BgaA is specific for galactose β-1,4-linked to glucose or GlcNAc [lactose or N-acetyllactosamine (LacNAc) motifs, respectively] found in glycoconjugates. The N-terminal region of BgaA comprising amino acid residues 138–993 has amino acid sequence identity with GH family 2 enzymes. Through detailed structural and functional analyses the molecular basis for the catalytic specificity of BgaA is defined and this activity is demonstrated as critical for the ability of pneumococci to utilize complex N-linked glycans as a carbon source and protect the bacterium from opsonophagocytic killing. Further analyses also revealed the presence of non-catalytic CBMs within the C-terminal region of BgaA that mediate adherence to host cell surface LacNAc and/or lactose.

However, fold prediction using the Phyre2 server, which does not rely on amino acid sequence similarity, distinguished two regions (XII and XV) with a high probability of adopting the β-sandwich fold common to many CBMs found in CAZymes. The two predicted CBMs were recombinantly produced and the polypeptides screened for binding to all commonly occurring monosaccharides by UV difference spectroscopy; only D-galactose gave a signature UV difference spectrum consistent with sugar binding. Subsequently, this approach was expanded to the relevant galactose-containing sugars LacNAc, lactose, galactopyranosyl-β-1,3-N-acetyl-D-glucosamine (lacto-N-biose), and galactopyranosyl-β-1,3-N-acetyl-D-galactosamine [Thomsen-Freidenreich (TF) epitope] and binding was only observed to LacNAc and lactose. Significantly, the CBMs only bound with significant affinity to sugars that are substrates for the catalytic domain. A single bound metal ion was modeled as Ca2+ on the basis of coordination geometry and B-factor analysis. The shallow LacNAc binding site sits at the apex of the β-fold opposite the N- and C-termini. Tryptophan 1514 lies directly beneath the glycoside bond and coplanar with the disaccharide thus providing CH-π interactions with both pyranose rings and a higher affinity for β-linked disaccharides than for galactose alone. This binding site architecture accommodates lactose and LacNAc, but would limit the recognition of other sugars terminating in β-linked galactose.

>[2x]LVPRGSHMNPNYDENSNQAFASATNDIDKNSHDRVDYLNDGDHSENRRWTNWSPTPSSNPEVSAGVIFRENGKIVERTVAQAKLHFFADSGTDAPSKLVLERYVGPGFEVPTYYSNYQAYESGHPFNNPENWEAVPYRADKDIAAGDEINVTFKAVKAKAMRWRMERKADKSGVAMIEMTFLAPSE>LKEAQNTCAMLTTFNEVDMSNIQEMRARHKDAFLKKHNLKLGFMSAFVKASAFALQEQPVVNAVIDDATKEVVYRDYIDISVAVATPRGLVVPVIRNVETMNYADIERTINELGEKARKNELAIEDMDGGTFTISNGG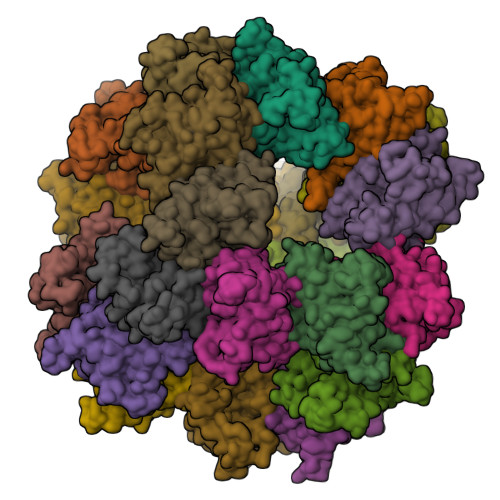VFGSLFGTPIINPPQSAILGMHGIFDRPVAVGGKVEVRPMMYVALTYDHRLIDGREAVTFLRKIKAAVEDPRVLLLDL[24x]> GGACCUCGCAAGGGUAUCAUGGCGGACGACCGGGGUUCGAACCCCGGAUCCGGCCGUCCGCCGUGAUCCAUGCGGUUACC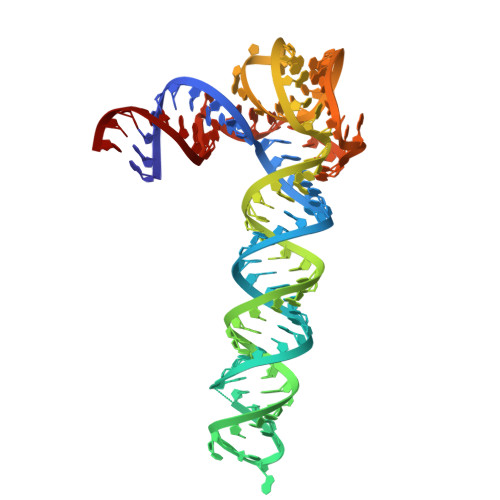GCCCGCGUGUCGAACCCAGGUGUGCGAGGUCC> NDVARGIVKADVAQSSYGLYGQGQIVAVADTGLDTGRNDSSMHEAFRGKITALYALGRTNNANDTNGHGTHVAGSVLGNGSTNKGMAPQANLVF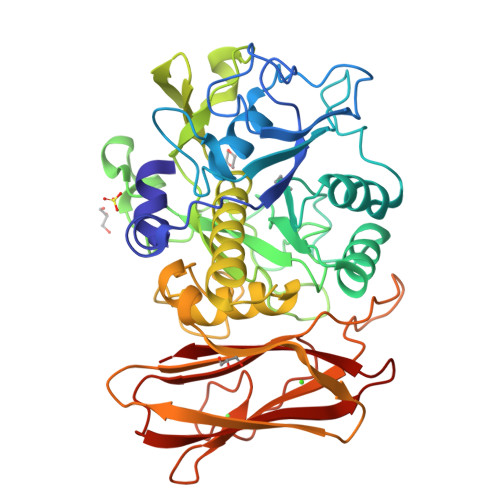QSIMDSGGGLGGLPSNLQTLFSQAYSAGARIHTNSWGAAVNGAYTTDSRNVDDYVRKNDMTILFAAGNEGPNGGTISAPGTAKNAITVGATENLRPSFGSYADNINHVAQFSSRGPTKDGRIKPDVMAPGTFILSARSSLAPDSSFWANHDSKYAYMGGTSMATPIVAGNVAQLREHFVKNRGITPKPSLLKAALIAGAADIGLGYPNGNQGWGRVTLDKSLNVAYVNESSSLSTSQKATYSFTATAGKPLKISLVWSDAPASTTASVTLVNDLDLVITAPNGTQYVGNDFTSPYNDNWDGRNNVENVFINAPQSGTYTIEVQAYNVPVGPQTFSLAIVN>MSNCQYKIYPPLGIARVGNGPAIKPLSLSTPEVPWAHLYDTNVQYLVTQQELEQLLEEAFGGNVINEISQIKTKLDERKAEKFKQEEIETITGLLGLSHLVPQQQLSRSLDNLELKSTKDSDDIVQQIKGALLKVLSDHYLHAVKKQAQNFYIYKCDEQGNPVEKLKLTDGDKVTWRVEVANKKSFWYDYNNALDLSLHTQGSGNLSKNVSKHRLAPAMTAKRRNPNVITNSLRKQLVISSQGSVSSDNNTQVPLRGKFPANEPDTNNRLSDLLNLQERHNVLQGSIECDNEGVLRFYAGNGISQALSPSSLNTDFADNSNWFDDICDGRVTAVVELKNGDTFEIQDEQSSAWVATTPPDYAPQIEPIVTMYDMVSGAALKEQDLDNLTTQFSDVFPILYRLYRMQWVNQADFTDNAVNTQIRELNSELGFAQLLDNSASAKSLREGIFNQFRNPLFDQDIDVDDPGQSSNEWVSNSRIIPSKDETNIAAKPATSSLKLPFYPNDGIDYPGSPVQWFAIPPFMYQHLQNWAAGDFSVTQVEKESANTIEELGLFYSEQFKNSPNSALLC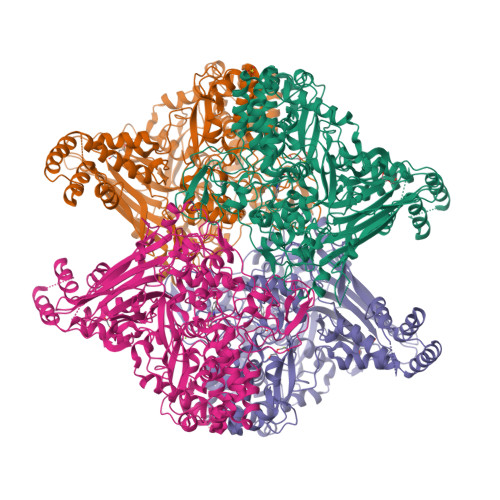ARGALDALYGGGFHPGVELTWPMRHNLIYSQNDYVSSVTPEINLLGLREFRLKQDLQGLNSPNMYQDFGHVIAVDNVTASIDPNSDAAWLWRSTPGDLTKWMGIPWQSDAASCQAVYTPEDFPIPSWWAANLPVHVLPLARYNKFKDSQSADLPEINGMTHSIAQGMSEETFEHLRLEQFSQRLDWLHTADLGFVGYHAEGGYTNGLIQMVSQWKNMAMVMARPVENPGSSGIPNVVYVAYSQADKD[4x]6-[(8R)-2-({[(3,5-dimethyl-1,2-oxazol-4-yl)methyl](methyl)amino}methyl)-6,7-dihydropyrazolo[1,5-a]pyrazin-5(4H)-yl]pyrimidin-4-amine | C18 H24 N8 O | 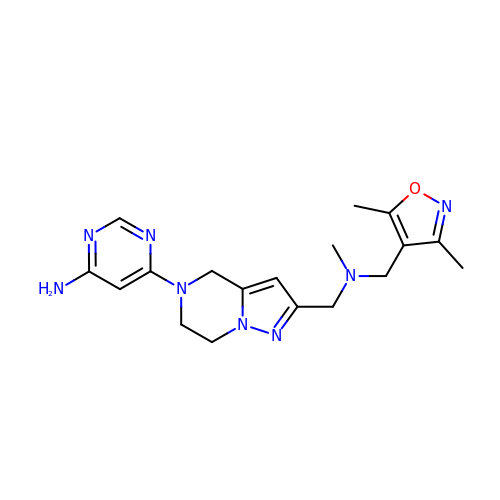UIAMVAYKSCWAMB-UHFFFAOYSA-N>[4x]SAEELLRRSREYLKKVALIQLVIAFVFLILLILLSWRSEELIRELEEKGAASEAELARMKQQHMTAYLQAALTAWEIISKSVIALLLLQQNQLNLELNTDTDKNVAEELLRRSREYLKKVA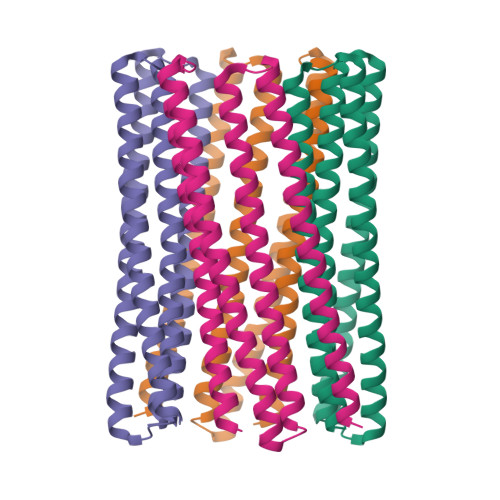LIQLVIAFVFLILLILLSWRSEELIRELEEKGAASEAELARMKQQHMTAYLQAALTAWEIISKSVIALLLLQQNQLNLELRH> GTMEELLTSLQKKCGTECEEAHRQLVCALNGLAGIHIIKGEYALAAELYREVLRSSEEHKGKLKTDSLQRLHATHNLMELL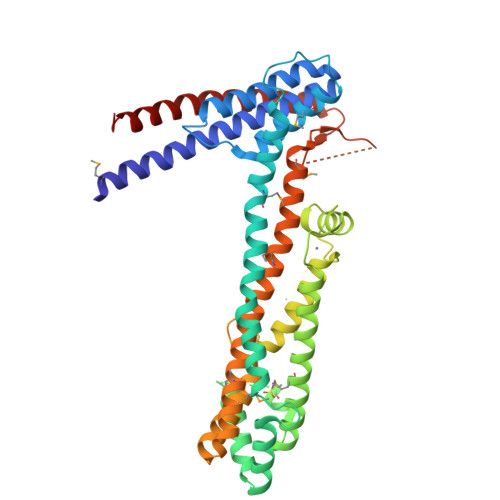IARHPGIPPTLRDGRLEEEAKQLREHYMSKCNTEVAEAQQALYPVQQTIHELQRKIHSNSPWWLNVIHRAIEFTIDEELVQRVRNEITSNYKQQTGKLSMSEKFRDCRGLQFLLTTQMEELNKCQKLVREAVKNLEGPPSRNVIESATVCHLRPARLPLNCCVFCKADELFTEYESKLFSNTVKGQTAIFEEMIEDEEGLVDDRAPTTTRGLWAISETERSMKAILSFAKSHRFDVEFVDEGSTSMDLFEAWKKEYKLLHEYWMALRNRVSAVDELAMATERLRVRDPREPKPNPPVLHIIEPHEVEQNRIKLLNDKAVATSQLQKKLGQLLYLTNLEK>SPSLDNPTPFPNLGPSENPLKRLLVPGEEWEFEVTAFYRGRQVFQQTISCPEGLRLVGSEVGDRTLPGWPVT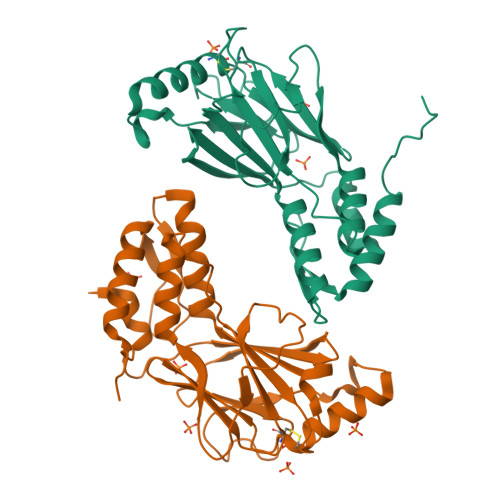LPDPGMSLTDRGVMSYVRHVLSCLGGGLALWRAGQWLWAQRLGHCHTYWAVSEELLPNSGHGPDGEVPKDKEGGVFDLGPFIVDLITFTEGSGRSPRYALWFCVGESWPQDQPWTKRLVMVKVVPTCLRALVEMARVGGASSLENTVDLHISNSHPLSLTSDQYKAYLQDLVEGMDFQGPGES[2x]>GPGSMVQSERRRLGVMGGTFDPIHNGHLVAASEVADRFALDEVIFVPTGQPWQKQGRKVSPAEHRYLMTVIATASNPRFTVSRADIDRGGATYTVDTLTDLRTAHPDADLYFITGADALASILSWENWEQLFTLAKFIGVSRPGYELSSDHIAHAELPPDGLSLVEVPALAISSTDCRIRAGQARPIWYLVPDG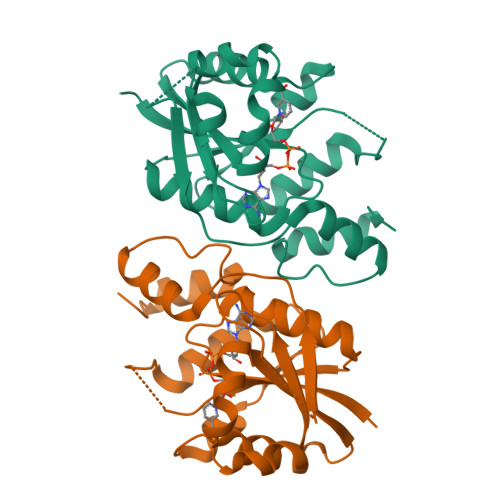VVQYVAKHRLYSGNKGNQGGLA[4x]> MASMKKSTENESTNYQYKIQELRKLLKS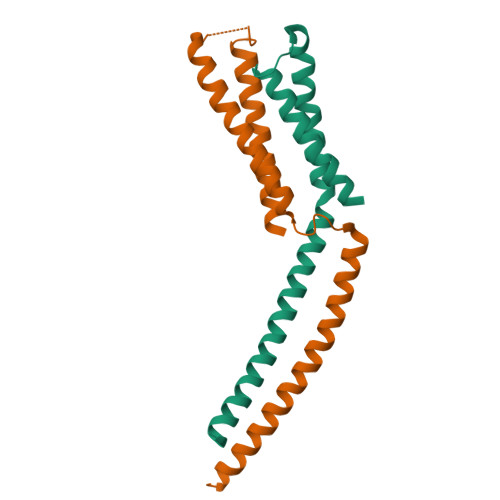LLLNYLELIGVLSINPDMYERKVENIRTILVNIHHLLNEYRPHQSRESLIMLLEEQLEYKRGEIREIEQVCKQVHDKLTS;> MTDRMTQLQICLDQMTEQFCATLNYIDKNHGFERLTVNEPQMSDKHATVVPPEEFSNTIDELSTDIILKTRQINKLIDSLPGVDVSAEEQLRKIDMLQKKLVEVEDEKIEAIKKKEKLMRHVDSMIEDFVDG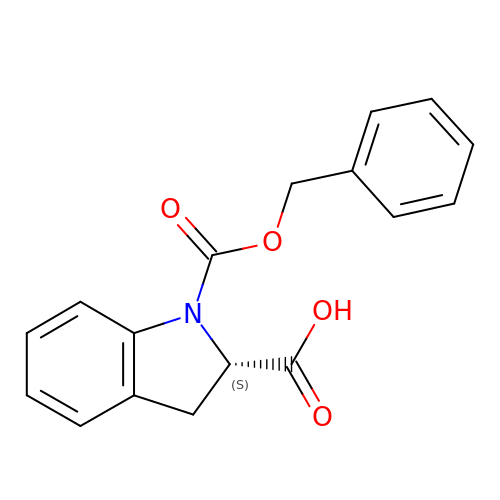(2S)-1-[(benzyloxy)carbonyl]-2,3-dihydro-1H-indole-2-carboxylic acid | C17 H15 N O4 | BSOYWTITVKXHLM-HNNXBMFYSA-N>[4x]MGSSHHHHHHSQDPNSSSMTLGHMVQKAKESSGDVTPKKYNIFLASKPVDGDRKWLDVTNKYTNDVAAKVPQATHKDI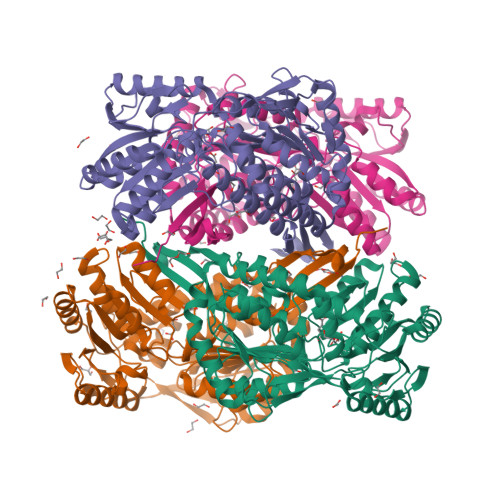DDAIDAAVAAAPAMAAMGAYERKAVLEKVVAELKNRFEEIAQTLTMESGKPIKDARGEVTRTIDTFQVAAEESVRIYGEHIPLDISARNKGLQGIVKKFPIGPVSMVSPWNFPLNLVAHKVAPAIAVGCPFVLKPASRTPLSALILGEILHKIEELPLGAFSILPVSREDADMFTVDERFKLLTFTGSGPIGWDMKARAGKKKVVMELGGNAPCIVDDYVPDLDYTIQRLINGGFYQGGQSCIHMQRLYVHERLYDEVKEGFVAAVKKLKMGNPFEEDTYLGPMISESAAKGIEDWVKEAVAKGGKLLTGGNRKGAFIEPTVIEDVPIEANARKEEIFGPVVLLYKYSDFKEAVKECNNTHYGLQSGIFTKDLNKAFYAFEHMEVGGVILNDSPALRVDSQPYGGLKDSGIQREGVKYAMDDMLETKVLVMRNVGTL>[2x]AESLPDLKIEKLDEGVYVHTSFEEVNGWGVVPKHGLVVLVNAEAYLIDTPFTAKDTEKLVTWFVERGYKIKGSISSHFHS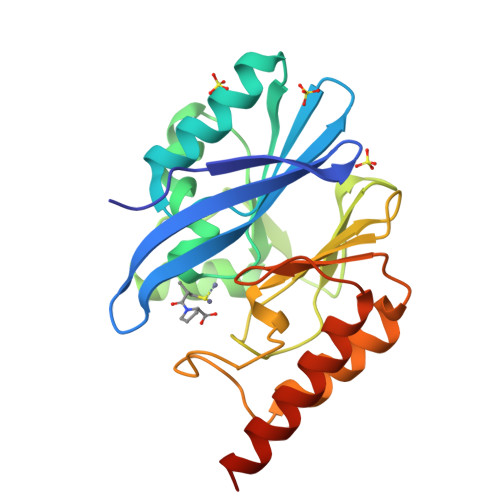DSTGGIEWLNSRSIPTYASELTNELLKKDGKVQATNSFSGVNYWLVKNKIEVFYPGPGHTPDNVVVWLPERKILFGGCFIKPYGLGNLGDANIEAWPKSAKLLKSKYGKAKLVVPSHSEVGDASLLKLTLEQAVKGLNESKKPSKPSN2-[(5-tert-butyl-2-methyl-phenyl)sulfonylamino]benzoic acid | C18 H21 N O4 S | 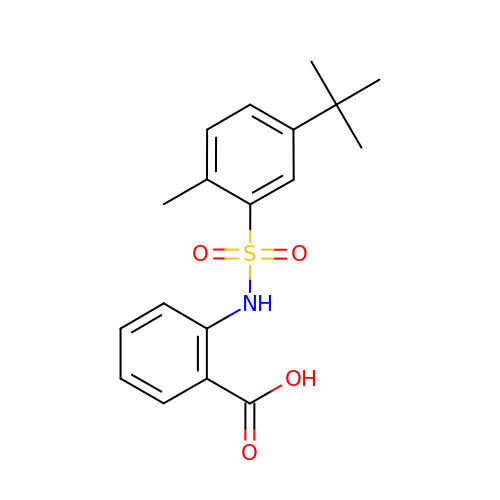FUWMRGQUYIVRDW-UHFFFAOYSA-N> MSAKDERAREILRGFKLNWMNLRDAETGKILWQGTEDLSVPGVEHEARVPKKILKCKAVSRELNFSSTEQMEKFRLEQKVYFKGQCLEEWFFEFGFVIPNSTNTWQSLIEAAPESQMMPASVLTGNVIIETKFF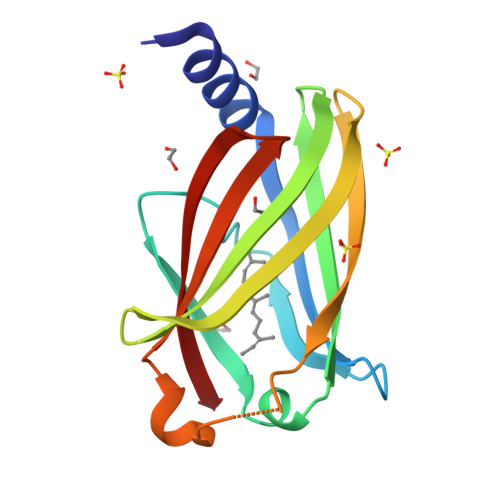DDDLLVSTSRVRLFYV> DVQINIRNNVYIPPCTINNGQNIVVDFGNINPEHVDNSRGEVTKTISISCPYKSGSLWIKVTGNTMGGGQNNVLATNITHFGIALYQGKGMSTPLTLGNGSGNGYRVTAGLDTARSTFTFTSVPFRNGSGILN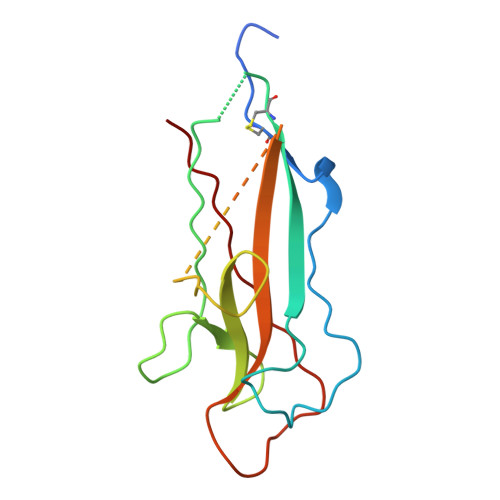GGDFRTTASMSMIYN>XGEFAQAVKEYAKAVKEYAYAVKEYA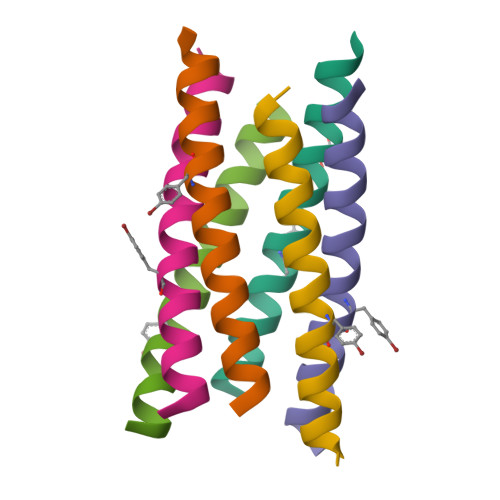QAVKGX[6x]>[180x]MAVAVGMIETLGFPAVVEAADAMVKAARVTLVGYEKIGTGRVTVIVRGDVSEVQASVSAGTESVKRVNGGQVLSTHIIARPHENLEYVLPIRYTEEVEQFREGVG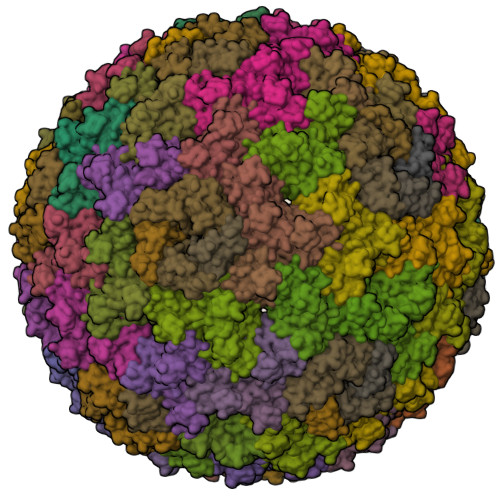TPRNITRQ;>MQMAKVCGTVVGTQKLPSMTGVKLLLLQFIDANGELLPKYEVAADPVGAGLGEWVLVNRGSAARQTEYHQNRPLDAMVVAIIDTVTVNNRRLYGEGSWSHPQFEK[60x]> FSIAVTGATGQLGGLVIQHLMAAVPASQIIAIVRNVEKASTLADQGVEVRHGDYNQPESLQKAFAGVSKLLFISGPHYDNTLLIVQHANVVKAARDAGVKHIAYTGYAFAEESIIPLAHVHLATEYAIRTTNIPYTFLRNALYTDFFVNEGLRASTESGAIVTNAGSGIVNSVTRNELALAAATVLTEEGHENKTYNLVSNQPWTFDELAQILSEVSGKK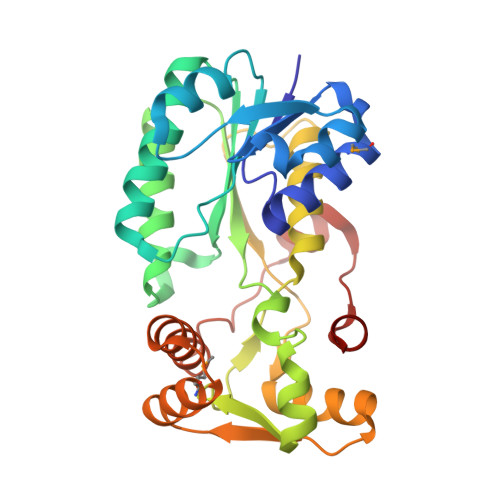VVHQPVSFEEEKNFMVNAGVPEPFAEITAAIYDAISKGEASKTSDDLQKLIGSLTPLKETVKQALKM>[2x]GPGDPHTYEDPNQAVLKFTTEIHPSCVTRQKVIGAGEFGEVYKGMLKTSSGKKEVPVAIKTLKAGYTEKQRVDFLGEAGIMGQFSHHNIIRLEGVISKYKPMMIITEYMENGALDKFLREKDGEFSVLQLVGMLRGIAAGMKYLANMNYVHRDLAARNILVNSNLVCKVSDFGLSRVLEDDPEATYTTS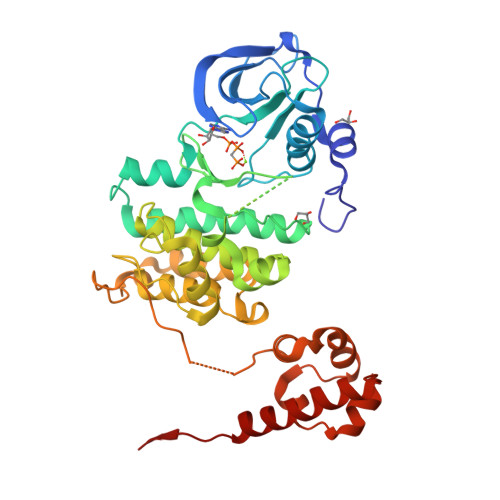GGKIPIRWTAPEAISYRKFTSASDVWSFGIVMWEVMTYGERPYWELSNHEVMKAINDGFRLPTPMDCPSAIYQLMMQCWQQERARRPKFADIVSILDKLIRAPDSLKTLADFDPRVSIRLPSTSGSEGVPFRTVSEWLESIKMQQYTEHFMAAGYTAIEKVVQMTNDDIKRIGVRLPGHQKRIAYSLLGLKDQVNTVGIPI>MAHHHHHHMSFSEWKTQPGAVFAASPVIPVIVIKELEDALPLAEALFAGGIHVLEVTLRTPVAIKALELLINTFPDELIGAGTVITPGQFHDVVAAGARFAISPGQTRELLIAGQKSEIPLIPGVASVSELMEGLGMGYNHFKFFPAAAAGGIPMLKAISGVFPQVKFCPTGGINSKNYEEYLCLPNVACVGGSWIVPEEAIKNHNWSLITELCMAVSS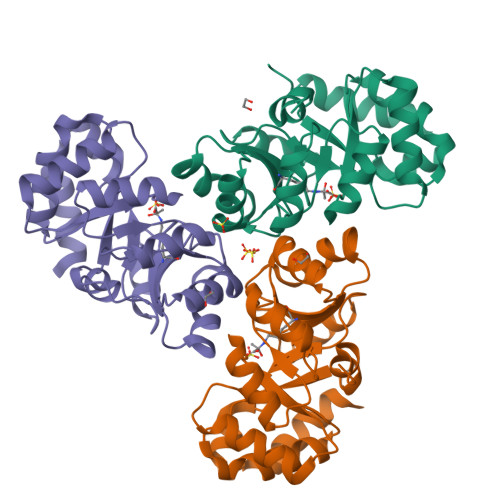QKRELCSQN[3x]>[2x]SVAILQKRDHEGFGFVLRGAKAE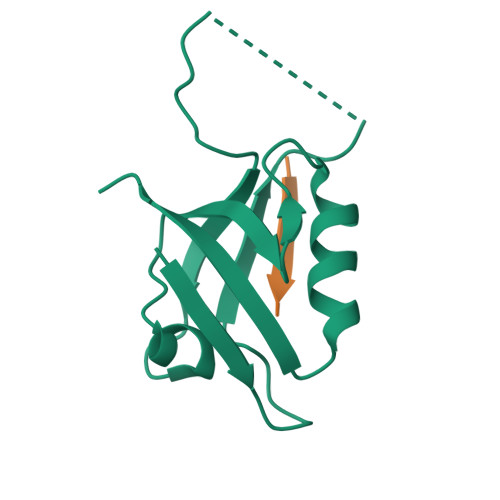TPIEEFTPTPAFPALQYLESVDVEGVAWKAGLRTGDFLIEVNGVNVVKVGHKQVVGLIRQGGNRLVMKVVSVT;>XDLQTSI[2x]>MKLFTGLVFCSLVLGVSSEWYSFLGEAAQGAWDMWRAYSDM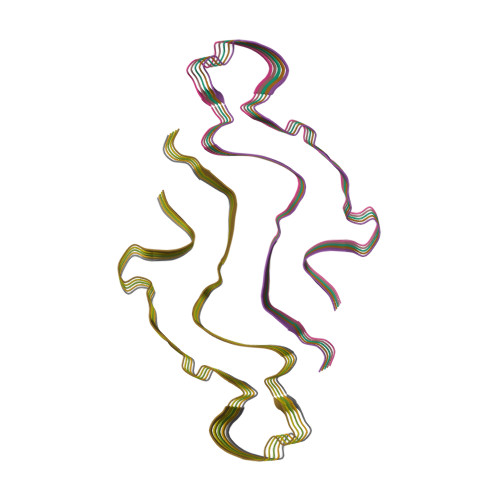REANYIGADKYFHARGNYDAAQRGPGGAWAAKVISDARENSQRVTDFFRHGNSGHGAEDSKADQEANEWGRSGKDPNHYRPEGLPDKY[10x]> KETAAAKFERQHMDS;> NYCNQMMKSRNLTKDRCKPVNTFVHESLADVQAVCSQKNVACKNGQTNCYQSYST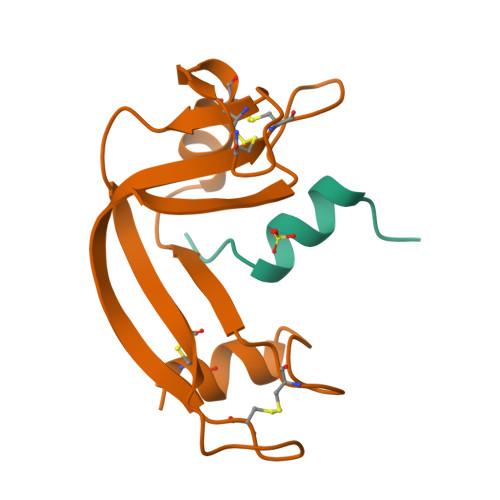MSITDCRETGSSKYPNCAYKTTQANKHIIVACEGNPYVPVHFDASV SufS is a pyridoxal-5′-phosphate–dependent enzyme that uses cysteine to generate alanine and an active-site persulfide (C364-S-S-). The SufS persulfide is protected from external oxidants/reductants and requires the transpersulfurase, SufE, to accept the persulfide to complete the SufS catalytic cycle. The β-latch contains four key components: the α6 helix, a glycine-rich loop, a β-hairpin, and a cis-proline. R92 and E96 (E. coli numbering) form cross-dimer electrostatic interactions with the α6 helix of the adjacent monomer, and N99 forms hydrogen bonds to the backbone amide and carbonyl of G251 in the glycine-rich loop.

We generated variants of SufS with either alanine or aspartate at position N99 and solved the crystal structures of the resulting proteins. Alteration of N99 results in significant, but localized, perturbations in components of the β-latch structural element. The most drastic effect is seen in the N99D SufS structure. In this structure, electron density is missing for residues 248 to 268, which includes the glycine-rich loop (G251-S254) and the β-hairpin (I256-T266). Additional perturbations are seen for residues R92 and E96 on the α6 helix. In the N99D SufS structure, the loss of density for the glycine-rich loop and the β-hairpin suggests increased solvent access to the active-site persulfide. In the absence of TCEP (open symbols), both WT and N99D SufS exhibit near identical alanine production kinetics to the WT enzyme in the presence of TCEP. Results for this experiment demonstrate that N99D SufS no longer inhibits the active-site persulfide from reacting with TCEP, consistent with the model that a key biological role of the β-latch is to shield the active-site persulfide from off-pathway reactions. When cysteine is added to N99D SufS, a rapid decrease of ∼50% is seen at ∼420 nm with a corresponding increase at ∼340 nm, similar to the results with the WT enzyme. However, the species do not persist, and the initial 420 nm absorbance state is regained after only 10 to 15 min rather than the 2-h time frame for the wildtype enzyme.

> MIFSVDKVRADFPVLSREVNGLPLAYLDSAASAQKPSQVIDAEAEFYRHGYAAVHRGIHTLSAQATEKMENVRKRASLFINARSAEELVFVRGTTEGIDLVANSWGNSNVRAGDNIIISQMEHHANIVPWQMLCARVGAELRVIPLNPDGTLQLETLPTLFDEKTRLLAITHVSNVLGTENPLAEMITLAHQHGAKVLVDGAQAVMHHPVDVQALDCDFYVFSGHKLYGPTGIGILYVKEALLQEMPPWEGGGSMIATVSLSEGTTWTKAPWRFEAGTPNTGGIIGLGAALEYVSALGLNNIAEYEQNLMHYALSQLESVPDLTLYGPQNRLGVIAFNLGKHHAYDVGSFLDNYGIAVRTGHHCAMPLMAYYNVPAMCRASLAMYNTHEEVDRLVTGLQRIHRLLG> 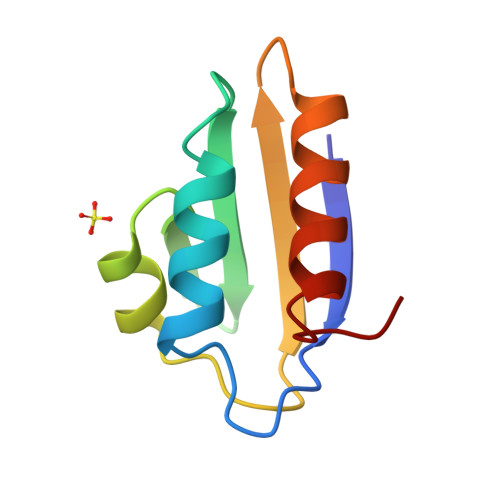AKFSAIITDKVGLHARPASVLAKEASKFSSNITIIANEKQGNLKSIMNVMAMAIKTGTEITIQADGNDADQAIQAIKQTMIDTALIQG>AVSLDRTAAVFDGSEKSMTLDISNDNKQLPYLAQAWIENENQEKIITGPVIATPPVQRLDPGAKSMVRLSTTPDISKLPQDRESLFYFNLREIPPRSEKANVLQIALQTKIKLFYRPAAIKTRPNEVWQDQLILNKVSGGYRIENPTPYYVTVIGLGGSEKQAEEGEFETVMLSP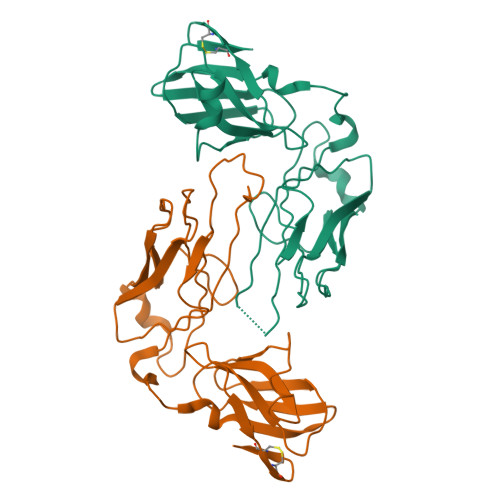RSEQTVKSANYNTPYLSYINDYGGRPVLSFICNGSRCSVKKEK[2x]> DPPPSETHKLVVVGGGGVGKSALTIQFIQSYFVSDYDPNIEDSYTKICSVDGIPARLDILD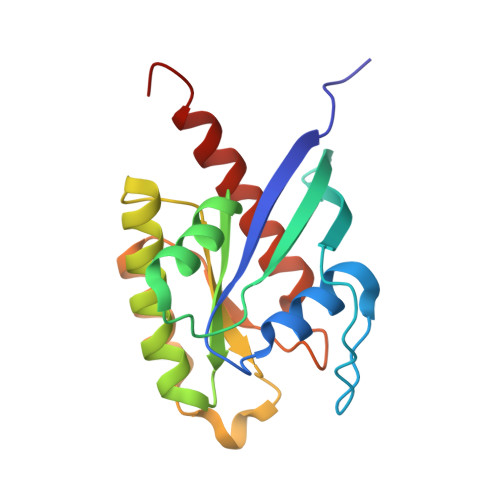TAGQEEFGAMREQYMRAGHGFLLVFAINDRQSFNEVGKLFTQILRVKDRDDFPVVLVGNKADLESQRQVPRSEASAFGASHHVAYFEASAKLRLNVDEAFEQLVRAVRKYQEQELPPS> SFFFLSFHISNLQFNSSLEDPSTDYYQELQRDISEMFLQIYKQGGFLGLSNIKFRPG;> SVVVQLTMAFREGTINVHDVETQFNQYKTEAASRYNLTISDVSV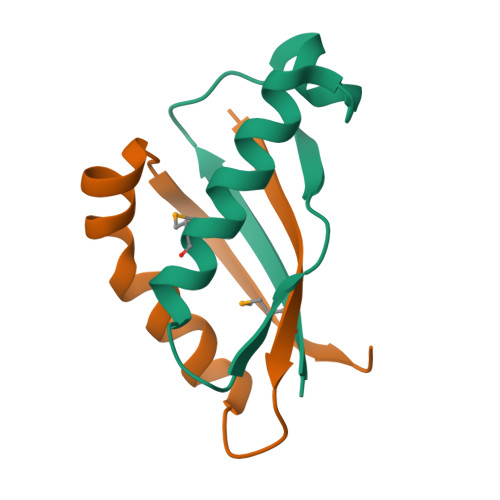SDVPFPFSAQS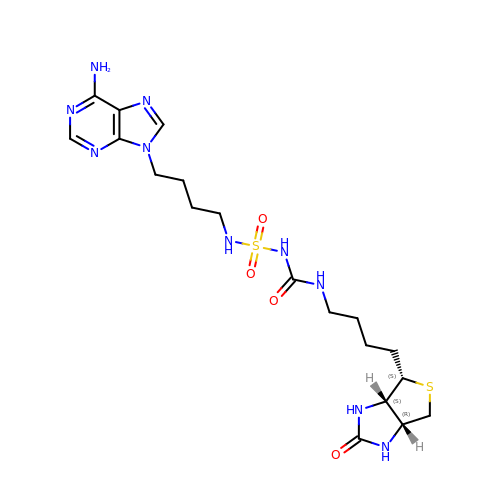1-[4-(6-aminopurin-9-yl)butylsulfamoyl]-3-[4-[(4~{S})-2-oxidanylidene-1,3,3~{a},4,6,6~{a}-hexahydrothieno[3,4-d]imidazol-4-yl]butyl]urea | C19 H30 N10 O4 S2 | NMZPYNDZFONMFP-IHRRRGAJSA-N>MKRVITYGTYDLLHYGHIELLRR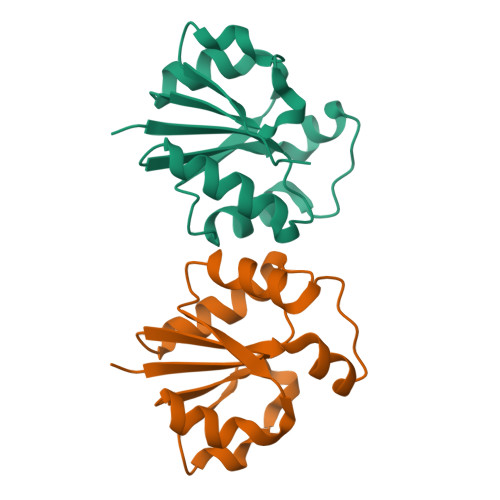AREMGDYLIVALSTDEFNQIKHKKSYYDYEQRKMMLESIRYVDLVIPEKGWGQKEDDVEKFDVDVFVMGHDWEGEFDFLKDKCEVIYLKRTEGISTTKIKQELYGKDAK[4x]>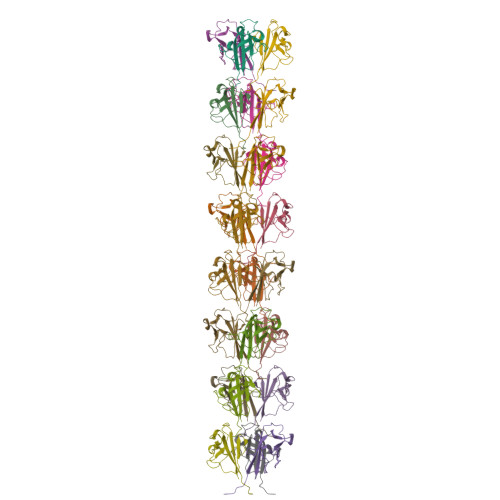[24x]MPIIQPFMASRRFTSTLGAGTGTGAAFAIAATACLNDAGTTATAFPTFTYYNLYVNGILQPSVNSSVTTGPTGAITIPGGDALDGGIPITIEFIVT> IVGGYTCEENSLPYQVSLNSGSHFCGGSLISEQWVVSAAHCYKTRIQVRLGEHNI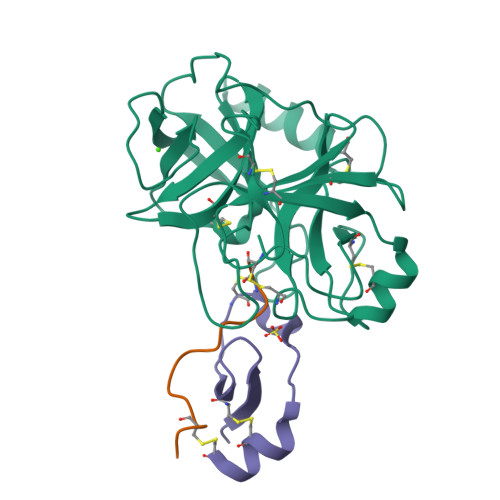KVLEGNEQFINAAKIIRHPKYNRDTLDNDIMLIKLSSPAVINARVSTISLPTAPPAAGTECLISGWGNTLSFGADYPDELKCLDAPVLTQAECKASYPGKITNSMFCVGFLEGGKDSCQRDAGGPVVCNGQLQGVVSWGHGCAWKNRPGVYTKVYNYVDWIKDTIAANS;> KAVCSQEAMTGPCR;> MPRWYFDLSKGKCVRFIYGGCGGNRNNFESEDYCMAVC> GAGEARLEEAVNRWVLKFYFHEALRAFRGSRYGDFRQIRDIMQALLVRPLGKEHTVSRLLR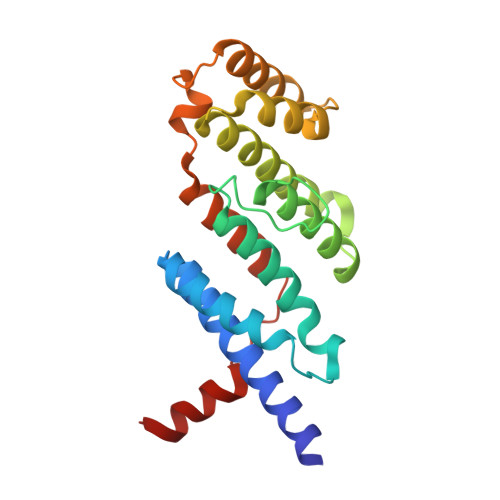VMQCLSRIEEGENLDCSFDMEAELTPLESAINVLEMIKTEFTLTEAVVESSRKLVKEAAVIICIKNKEFEKASKILKKHMSKDPTTQKLRNDLLNIIREKNLAHPVIQNFSYETFQQKMLRFLESHLDDAEPYLLTMAKKALK>MDPEGLALLLPPATLATLADSWLREDCPGLNPVALVTGAAPSQAVLWAKSPGILAGRPFFDAIFAQVNCQVSWFLPEGSKLVPVAKVAEVRGPAHCLLLGERVALNMLARCSGVASAAAT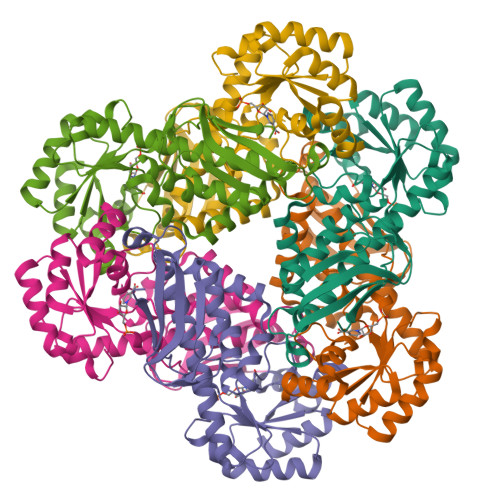AVETARGTGWAGHVAGTRKTTPGFRLVEKYGLLVGGATSHRYDLGGLVMVKDNHVVAAGGVKQAVQGARRAANFALKVEVECSSLQEALEAAEAGADLVLLDNFRPEELHPTAAALKAQFPTVGVEASGGVTLDNLPQFCGPHIDVISLGMLTQAAPALDFSLKLFAE[2x]> MFFELEDIKRRHSLYWDIYNVQGWVRRPDSTLYNNVKRGVTAGVVASLVQENITALVENCKLLATKYEKPQNLRQAATFMKEVFKLENYRKAVWNRSQYALCIGTFDIGARLATFRWLNNGWQRVFAGFEFNFVRKIPTTMLAALFTAPFSVPFELA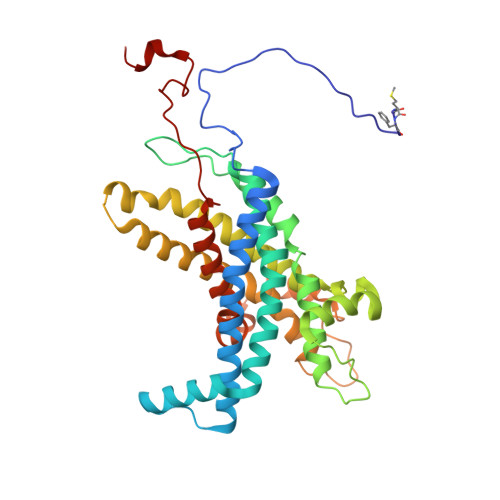RMAYYGDKTFPKELQRGYSSYLSALARIPFEEGPYFLFKNSFPLIIRNFFQTFTLFYTYDFLKDKASFAWRVGEQNEYACKMIIAGISTYLAAVFSYPWMVTREMVDFWPKVPGAPCTFNGNYRKAAVWIWYHEFSGNYFAGFFTKYFWKASPGMFLTLMLADKVGLFDQTTVDNFGGAGNNSWEDTFV>HNKVRTCWNEGRPALAGWLQLPGTLHAEALARLDYDAVVIDMQASPIDFGQVAPMLIAIELGGAEPFVRTQVNDPSDIMKLLDAGAYGIIAPMVNTRAEAQTLASALHYSPRGLRSFGPRRPSLRYGSGYLAQASETVVGLAMIETREALANIDEILSVDGIDGVFIGPTDLALDLGHAPLVDTEEAEVVSAIAHVRERAHAAGKRVGIFCGSGGFARVKLAEGFDFVTAAP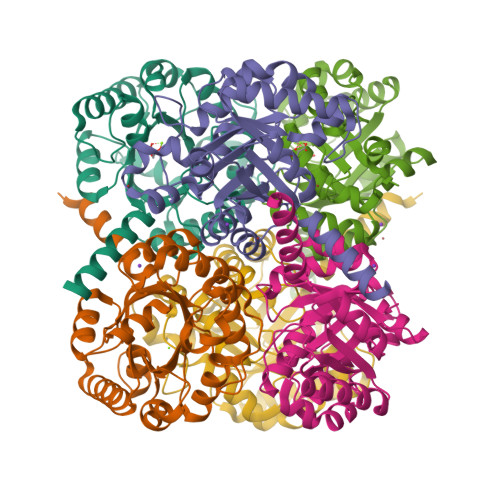DLAMLSAAARQVIADARAL[2x]> TRYIPDEAD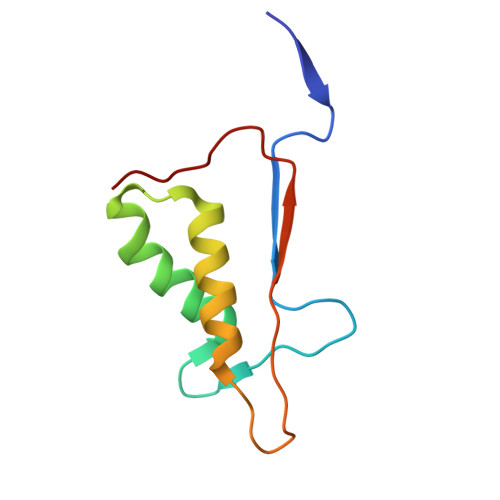FLLGMATVNNCVSYRNPAEGTWYIQSLCQSLRERCPRGDDILTILTEVNYEVSNKDDKKNMGKQMPQPTFTLRKKLVFPS> GHMSQSNRELVVDFLSYKLSQKGYSWSQFSDVEENRTEAPEETEAERETPSAINGNPSWHLADSPAVNGATGHSSSLDAREVIPESAVKQALREAGDEFELRYRRAFSDLTSQLHITPGTAYQSFEQVVNELFRDGVNWGRIVAFFSFGGALCVESVDKEMQVLVSR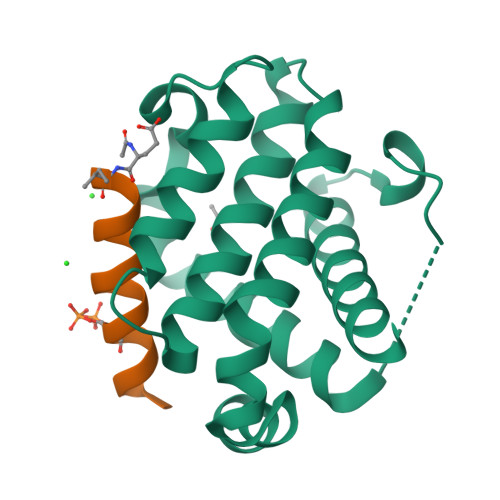IASWMATYLNDHLEPWIQENGGWDTFVDLYG;> XIWIAQELRRRGDSFNAYYAR> VLGGHECQPHSQPWQAALFQGQQLLCGGVLVGGNWVLTAAHCKKPKYTVRLGDHSLQNKDGPEQEIP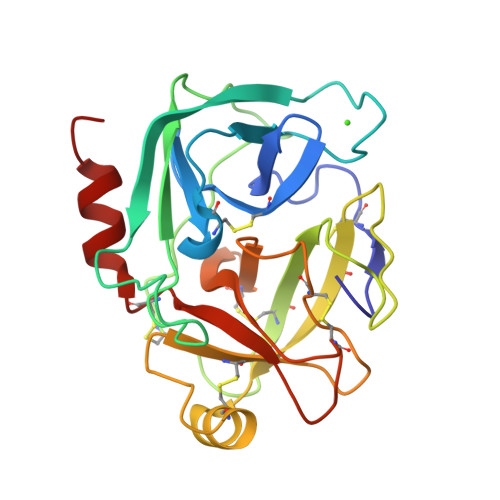VVQSIPHPCYNSSDVEDHNHDLMLLQLRDQASLGSKVKPISLADHCTQPGQKCTVSGWGTVTSPRENFPDTLNCAEVKIFPQKKCEDAYPGQITDGMVCAGSSKGADTCQGDSGGPLVCDGALQGITSWGSDPCGRSDKPGVYTNICRYLDWIKKIIGSKG Transfer RNA–guanine transglycosylase (Tgt, EC 2.4.2.29) catalyses the exchange of a specific guanine base in tRNA molecules by a substituted 7-deazaguanine. Bacterial Tgt functions as a homodimer in which the protomer consists of a (βα)8 barrel harbouring a Zn2+ binding subdomain close to the C-terminus. The reaction follows a ping-pong mechanism including a covalent Tgt⋅tRNA intermediate. Hence, in an attempt to generate a model system for the active site of human Tgt and to gain insights into the relevance of particular amino acids for substrate base selectivity, we adapted the Z. mobilis Tgt active site by site-directed mutagenesis in order to mimic that of the human enzyme.

Nucleobase mimetics endowed with bulky exocyclic substituents, however, generally constitute purely competitive inhibitors with respect to tRNA as their binding to the covalent Tgt·tRNA complex would sterically interfere with the tRNA sugar phosphate backbone.

> MVEATAQETDRPRFSFSIAAREGKARTGTIEMKRGVIRTPAFMPVGTAATVKALKPETVRATGADIILGNTYHLMLRPGAERIAKLGGLHSFMGWDRPILTDSGGFQVMSLSSLTKQSEEGVTFKSHLDGSRHMLSPERSIEIQHLLGSDIVMAFDEVTPYPATPSRAASSMERSMRWAKRSRDAFDSRKEQAENAALFGIQQGSVFENLRQQSADALAEIGFDGYAVGGLSGGEGQDEMFRVLDFSVPMLPDDKPHYLMGVGKPDDIVGAVERGIDMFDCVLPTRSGRNGQAFTWDGPINIRNARFSEDLKPLDSECHCAVCQKWSRAYIHHLIRAGEILGAMLMTEHNIAFYQQLMQKIRDSISEGRFSQFAQDFRARYFARNS>ELFRGVLQVSSNVLDCANDNWWCSLLDLDTSDWEPLTHTNRLMAIYLSSVASKLDFTGGPLAGCLYFFQVECNKFEEGYHIHVVIGGPGLNPRNLTVCVEGLFNNVLYHLVTGNVKLKFLPGMTTKGKYFRDGEQFIENYLMKKIPLNVVWCVTNIDGYIDTCISATFRRGACHAKKPRMTTAINDTSSDAGEPSGTGAEVVPFNGKGTKASIKFQTMVNWLCENRVFTEDKWKLVDFNQYTLLSSSHSGSFQIQSALKLAIYKATNLVPTSTFLLHADFEQVMCIKDNKIVKLLLCQNYDPLLVGQHVLKWIDKKCGKKNTLWFYGPPSTGKTNLAMAIAKSVPVYGMVNWNNENFPFNDVAGKSLVVWDEGIIKSTIVEAAKAILGGQPTRVDQKMRGSVAVPGVPVVITSNGDITFVVSGNTTTTVHAKALKERMVKLNFTVRCSPDMGLLTEADVQQWLTWCNAQSWDHYENWAINYTFDFPGINADALHPDLQTTPIVTDTSISSSGGESSEELSESSFFNLITPGACNTETPRSSTPIPGTSSGESLVGSPVSSEVVAASWEE[6x]

The main replication protein NS1 plays a critical role in cell cycle arrest, transactivation of viral and host genes, and replication and package of B19V genome. Based on its similarity to other parvoviral replication proteins, such as Rep72 of the adeno-associated virus (AAV), NS1 is predicted to contain one nuclease domain (Nuc, aa 1–176), one oligomerization domain (OD, aa 201–270), one SF3 helicase domain (SF3 HD, aa 271–501), and one zinc-binding domain (ZnD, aa 571–671). The SF3 HD domain of NS1 belongs to the SF3 helicase superfamily, which unwinds DNA with 3′→5′ polarity. Totally, four cryo-electron microscopy (cryo-EM) structures were determined, which revealed the detailed mechanisms for ATP binding and hydrolysis and DNA binding and unwinding by NS1.

To reveal how NS1 unwinds DNA, a DNA with overhangs at both ends, the overhang DNA-2, was designed and included in the cryo-EM sample. One ternary complex was determined at an overall resolution of 3.3 Å. Since the dsDNA region is disordered and only the ssDNA portion and AMPPNP are observed, the structure was termed as NS1_2-570/ssDNA/AMPPNP complex hereafter. Instead of dodecamer, NS1_2-570 exists as hexamer in the NS1_2-570/ssDNA/AMPPNP complex. The ssDNA mainly interacts with the SF3 HD domain with the 5′-end pointing toward the OD domain. In the NS1_2-570/ssDNA/AMPPNP structure, the ssDNA adopts B-form-like conformation; its backbone phosphate groups form several H-bond interactions with the side chains of Lys398 of NS1 protomers B–E. The side chains of Met399 of protomers B–E point toward the sugar puckers of ssDNA, forming hydrophobic stacking interactions. However, unlike the DNA-free structure, the SF3 HD domains adopt asymmetric assembly and tilt toward the central channel in the ssDNA-bound structure. Direct superposition showed that ssDNA binding also leads to large conformational change at the 393–407 region, which folds into a short α-helix in the DNA-free structure and a β-sheet in the DNA-bound structures, respectively. The side chain of Arg438 forms one H-bond interaction with the γ-phosphate of AMPPNP, and the β-phosphate interacts with the side chains of Lys320 and Gln391.> MPACSGLHAHADQQSSLLQLLAQRKGAYSGRPDINQQSRGFASSAGSDNSSSGQQAAGLESERLAPTTRLQDLVAGATERIAQKQVGTLGQLPEQLAAEAASLEHQLASSSGRSGHTHDLDGAGALADRLASAAAAGGPDGRAGGADGAAVTAGQRLLHNKYGYAALGGVVPDGGEMMAAAGPAAVLRSVTAAQ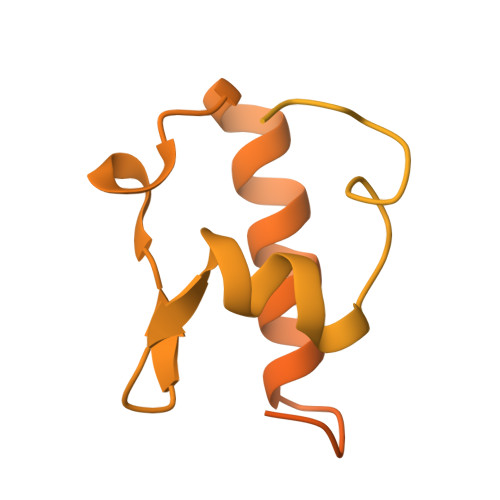PRLHPRRRFQPGQTYEPQDLNPYSSASPESRQRGVGVAVPRPSVAEVLEKADYKNVAFLTRWFLSPAGRLLPRRQTRLPVAVHKHVSRQVRLARHMGLIAGEARLDKTHVQALREVEAAQLLAGRLVAGAEAGAQQQAAAGAGAGAGAAPRQRYNELLDFGA> AMRQCAIYGKGGIGKSTTTQNLVAALAEM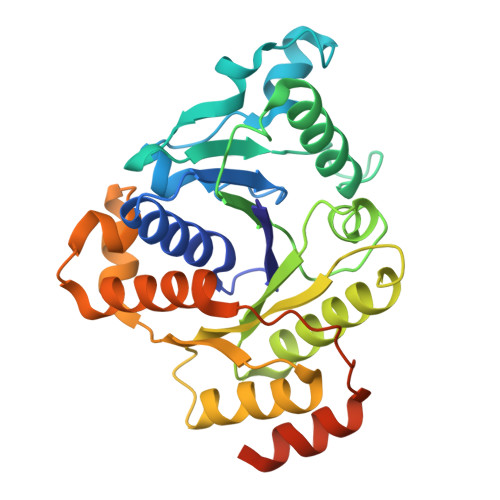GKKVMIVGCDPKADSTRLILHSKAQNTIMEMAAEAGTVEDLELEDVLKAGYGGVKCVESGGPEPGVGCAGRGVITAINFLEEEGAYEDDLDFVFYDVLGDVVCGGFAMPIRENKAQEIYIVCSGEMMAMYAANNISKGIVKYANSGSVRLGGLICNSRNTDREDELIIALANKLGTQMIHFVPRDNVVQRAEIRRMTVIEYDPKAKQADEYRALARKVVDNKLLVIPNPITMDELEELLMEFGIMEVEDESIVGKTAEEV>[4x]MGFKGVGTYEIVPYQAPSLNLNAWEGKLEPGAVVRTYTRGDKPSDNAKWQVALVAGSGDSAEYLIINVHSGYFLTATKENHIVST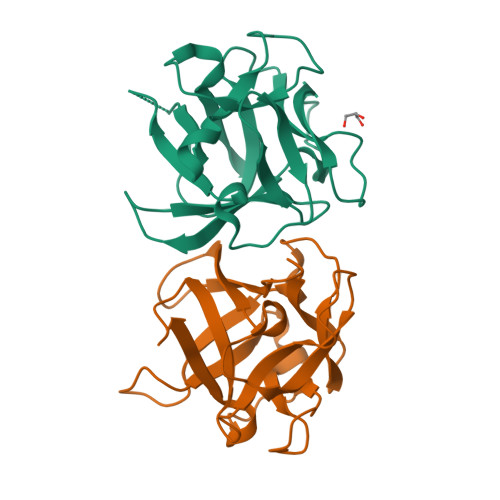PQISPTDPSARWTIKPATTHQYEVFTINNKVSELGQLTVKDYSTHSGADVLSASAKTADNQKWYFDAK> STEDEGEDPWYQKACKCDCQGGPNALWSAGATSLDCIPECPYHKPLGFESGEVTPDQITCSNPEQYVGWYSSWTANKARLNSQGFGCAWLSKFQDSSQWLQ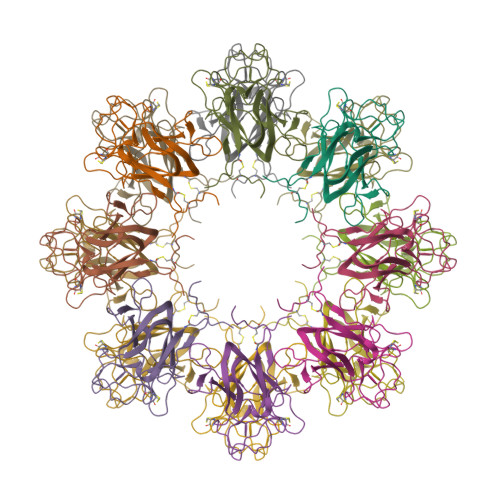IDLKEIKVISGILTQGRCDIDEWMTKYSVQYRTDERLNWIYYKDQTGNNRVFYGNSDRTSTVQNLLRPPIISRFIRLIPLGWHVRIAIRMELLECVSKCAHHHHHH>[8x]MATLRVHPEAQAKVDVFREDLCSKTENLLGSYFPKKISELDAFLKEPALNEANLSNLKAPLDIPVPDPVKEKEKEERKKQQEKEEKE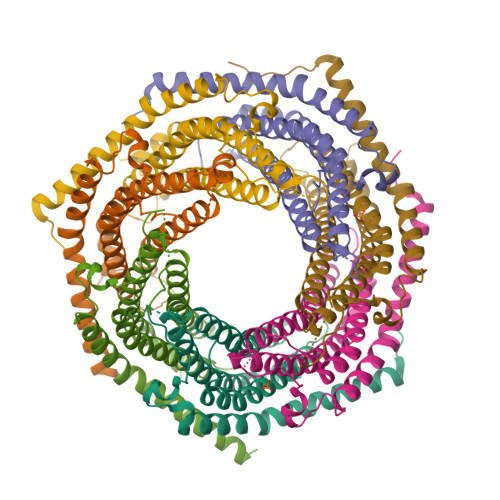EKKKGDEDDKGPPCGPVNCNEKIVVLLQRLKPEIKDVTEQLNLVTTWLQLQIPRIEDGNNFGVAVQEKVFELMTNLHTKLEGFHTQISKYFSERGDAVAKAAKQPHVGDYRQLVHELDEAEYQEIRLMVMEIRNAYAVLYDIILKNFEKLKKPRGETKGMIY;>MAKPCGVRLSGEARKQVDVFRQNLFQEADDFLCTFLPRKIISLSQLLQEDSLNVADLSSLRAPLDIPIPDPPPKDDEMETDKQEKKEVPKCGYLPGNEKLLALLALVKPEVWTLKEKCILVITWIQHLIPKIEDGNDFGVAIQEKVLERVNAVKTKVEAFQTTISKYFSERGDAVAKASKDTHVMDYRALVHERDEAAYGALRAMVLDLRAFYAELYHIISSNLEKIVNPKGEEKPSMY[6x]>MAPDLSGTWYVLEGDPGEHLVVEALGERLSGIWTSRELAEAFLAHHPHLGMRVSALESRALKEAYLRALGMLQV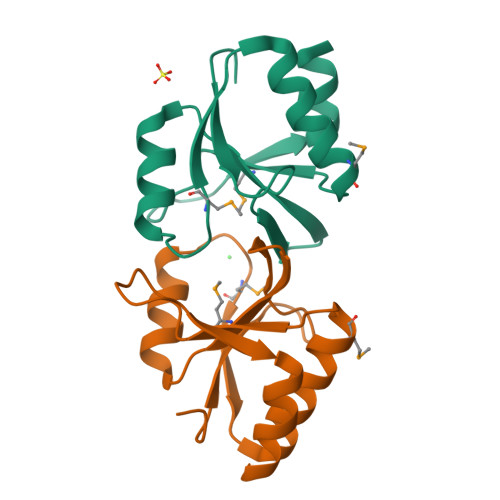EAVMVDYRPGTHRAQVARVKDLLEEVRRA[12x]>DLSQCDREPIHLLGGIQSHGVLLAFRGPDRLLEVVSANAQALLGRPPETLLGQPVGRVLPAEVLAQWEPLVARGSVRVVLPAGAYRALLHESDGLTVLELEPAELQPGMEETALEVVRRLVSPLAGVKGTQALLQTAADTVRALTGFDRVMVYRFDADWHGEVLAESKRGGMDGFLGMHFPATDIPVQARALYTRNPLRLIADARARPVPLLPPVVPALGRPLDLSNSALRSVSPVHLEYLRNMGVGASFSLSLLKEGVLWGLIACTHLEPLHISHERRRACEVLTQLLALQLSAEERAAEASEDAHRAALLGQLATAMGEGGTLEEVLEKESERVLALTGAAGVALLLGEEPLLVGCTPAQDEVEALVAWLATQPFQTSFHTDRLGTVYPPLAARADVAAGILAVRLAPAAARFAIWFRPEVARTISWAGNPRKPAEPEPGHQRLHPRGSFQAWEETVRDTSLPWKRADLGAAEGFRGAL[2x]

Phytochromes (PHYs) are red-light sensing enzymatic switches first discovered in plants, with homologs in the photosynthetic and nonphotosynthetic bacteria. PHYs are composed of a photosensory core module (PCM) and an effector, enzymatic domain. In bacteriophytochromes (BphPs), the PCM consists of three domains named PAS (Per ARNT Sim), GAF (cGMP phosphodiesterase/adenylyl cyclase/FhIA), and PHY (phytochrome-specific GAF-related) [Fig. 1(a)].1–5 The effector domain is typically a histidine kinase, covalently linked to a PHY domain, although other nonenzymatic output domains can be found. However, both proteins bind the same bilin chromophore and share a large amino acid sequence identity (38%).5,14,18 Biliverdin (BV) is an open-chain tetrapyrrole that is highly conjugated and allows for reversible photoconversion in BphPs between the red light absorbing (Pr, λmax 700 nm) and far-red light absorbing (Pfr, λmax 750 nm) states. Here, we report three crystal structures of the SaBphP2 photosensory core module (PCM), lacking the effector histidine kinase domain.

The reported structures are of a SaBphP2 PCM in the wild-type (wt) and mutant forms determined at 1.65 Å and 2.2 Å, respectively. The cryostructure of the His275Thr mutant is essentially identical to that of the wild-type, except at the location of the point mutation where the hydrogen bond to the ring D carbonyl is absent. The conserved Histidine, although absent in some myxobacterial BphPs such as SaBphP1, stabilizes the Pr state by forming a H-bond with the D-ring carbonyl and the Pfr state by forming a H-bond with the C-ring propionate. Serine is absent in the SaBphP2 wild-type protein, and likewise, the mutation His275Thr diminishes the Pr/Pfr photoactivity, possibly as there is no stabilizing amino acid for the D-ring and C-ring propionate in the Pr and Pfr states. Upon Z to E isomerization and by rotation of the D-ring about the C15=C16 double bond, the conserved Histidine 275 must move.> MHHHHHHHAVRASEISRVYEAYPEKKATLYFLVLGFLALIVGSLFGPFQALNYGNVDAYPLLKRLLPFVQSYYQGLTLHGVLNAIVFTQLFAQAIMVYLPARELNMRPNMGLMWLSWWMAFIGLVVFALPLLANEATVLYTFYPPLKGHWAFYLGASVFVLSTWVSIYIVLDLWRRWKAANPGKVTPLVTYMAVVFWLMWFLASLGLVLEAVLFLLPWSFGLVEGVDPLVARTLFWWTGHPIIYFWLLPAYAIIYTILPKQAGGKLVSDPMARLAFLLFLLLSTPVGFHHQFADPGIDPTWKMIHSVLTLFVAVPSLMTAFTVAASLEFAGRLRGGRGLFGWIRALPWDNPAFVAPVLGLLGFIPGGAGGIVNASFTLDYVVHNTAWVPGHFHLQVASLVTLTAMGSLYWLLPNLTGKPISDAQRRLGLAVVWLWFLGMMIMAVGLHWAGLLNVPRRAYIAQVPDAYPHAAVPMVFNVLAGIVLLVALLLFIYGLFSVLLSRERKPELAEAPLPFAEVISGPEDRR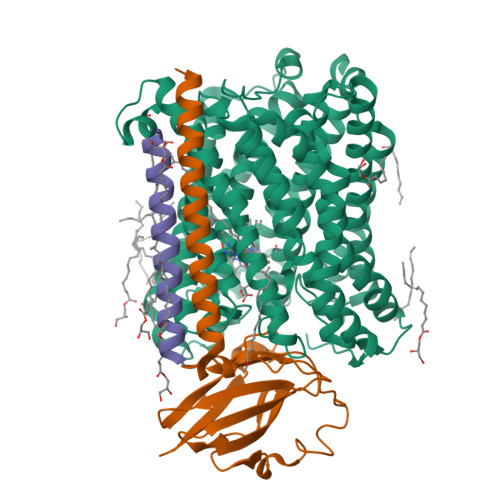LVLAMDRIGFWFAVAAILVVLAYGPTLVQLFGHLNPVPGWRLW;> MVDEHKAHKAILAYEKGWLAFSLAMLFVFIALIAYTLATHTAGVIPAGKLERVDPTTVRQEGPWADPAQAVVQTGPNQYTVYVLAFAFGYQPNPIEVPQGAEIVFKITSPDVIHGFHVEGTNINVEVLPGEVSTVRYTFKRPGEYRIICNQYCGLGHQNMFGTIVVKE;> MEEKPKGALAVILVLTLTILVFWLGVYAVFFARG> MADVVTEFGALTDYRKGGVEIIDDDPRNYVFSNVFEVAANAAPYERVAVGKNFEYVIESARAEGTSGWFSCAHDEFVLAMDGQIEVHLLKLDNSDAYVDPDSEGAVAIGEALPEGRKMGRIVLRRGHMALLPVG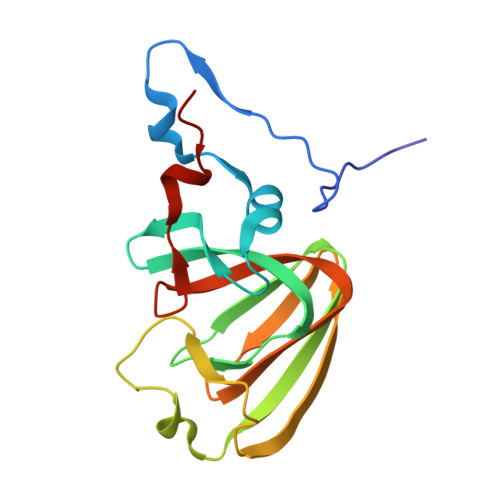AAYRFYAEQPAAMLFQSIEGAVTVQKWGEICQTEAA> SITSSLDVRPEIKQAVTVRPGMCGPGSLFVGQLGDWTWETVSAQCDTDVFAARDASGNPTYLAFYYFRVRGGRELHPGSLTFGDRLTVTSGCYDQGTESVLTLHRIDRAGSDDAQRPLDLHEFYERPRDGSLYVENFNRWVTRSAPGSNEDLVKSSPPGFRNDGLPQLPAAYSPRAVYREARTAHTFRALDEPGFRLLPDTVEVEHPVDIVRDVNGVGLL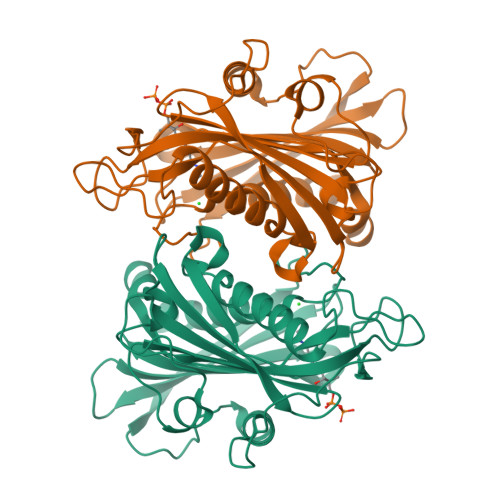YFASYFSMVDKAALALWRRLGRSDRAFLRRVVVDQQMCYLGNADLDSVLTLGARVRVSTETPGEELVDVVISDRDSGRVIAVSTLHTQHDAHDPKGEA>MASWSHPQFEKIEGRSMDNINLMPDEPTRFTPVFMDRMLEHAESLNASDITIQTGEPIFAEVYGRLLKITNRRLSNTELGDLINSIYGPNATTQLLSGKDIDTHYEFRPNRGVRYRYRVNATACLVEGHDAIQITLRTIPTTPPKLSTMNLPDNIIEAIAPQEGIVFITGATGSGKSTLLASIIRELIETSDSNRKVLTYESPIEFVYDEIETISAVVSQSEIPRHLPNFADGVRNALRRKPRLIMVGECRDAETISAALEAALTGHPVYTTLHTSGVAETMRRLVTSFSGEERLGRTIDILETIRLCIWQKLVPTVDERRVALREYLVFDEEVRDILLEGDPNEVTSATRKLVRQKG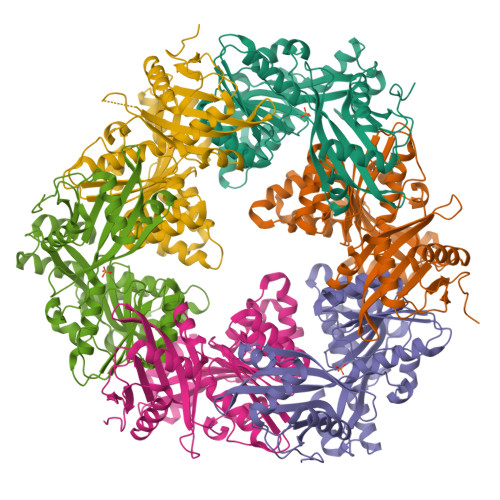QLMTWDAKMKFEQGIISERVYKLIIAGAKEYQQ[12x]>[3x]MGSSHHHHHHSQDPVSGTPDDGDIGLIIAVKRLAAAKTRLAPVFSAQTRENVVLAMLVDTLTAAAGVGSLRSITVITPDEAAAAAAAGLGADVLADPTPEDDPDPLNTAITAAERVVAEGASNIVVLQGDLPALQTQELAEAISAARHHRRSFVADRLGTGTAVLCAFGTALHPRFGPDSSARHRRSGAVELTGAWPGLRCDVDTPADLTAARQLGVGPATARAVAHR

Cofactor F420 is a deazaflavin that acts as a hydride carrier in diverse redox reactions in both bacteria and archaea. In the second branch, it has been hypothesized that a 2-phospho-l-lactate guanylyltransferase (CofC in archaea and the putative enzyme FbiD in bacteria) catalyzes the guanylylation of 2-phospho-l-lactate (2-PL) using guanosine-5ʹ-triphosphate (GTP), yielding l-lactyl-2-diphospho-5ʹ-guanosine (LPPG). Mass spectrometry (MS) and protein crystallography are used to demonstrate that PEP guanylylation is catalyzed by the FbiD/CofC enzymes that were previously thought to act upon 2-PL.

To understand the molecular basis of PEP recognition by Mtb-FbiD, we crystallized the protein and solved the structure by selenium single-wavelength anomalous diffraction (Se-SAD), and then used this selenomethionine-substituted structure to obtain the native FbiD structure by molecular replacement. The latter was then refined at 1.99 Å resolution (R/Rfree = 0.19/0.22). As expected, Mtb-FbiD adopts the same MobA-like nucleoside triphosphate transferase family protein fold as CofC: a central 7-stranded β-sheet (six parallel strands and one antiparallel), with α-helices packed on either side. FbiD has a cone-shaped binding cleft with a groove running across the base of the cone, formed by the C-terminal end of the central β-sheet. Moreover, we did not observe GTP binding in either our co-crystallization or differential scanning fluorimetry experiments. We speculate that the GTP binding site is not formed until FbiD/CofC interacts with FbiA/CofD, enabling catalysis to proceed through to formation of dehydro-F420-0.Potassium channels propagate electrical signals, maintain membrane potentials and facilitate numerous downstream cellular processes. KirBac3.1 adopts the canonical fold of a K+ channel, with inner and outer membrane-spanning helices supporting an inclined, shorter, pore helix that supports the signature selectivity filter. All feature an hourglass-like constriction at the intracellular opening, leading to the widespread conclusion that the canonical permeation gate at the helix bundle crossing is closed (or nearly so) in all Kir structures, whether determined by crystallography or single-particle cryo-EM. Thus, data presented here indicate that inward rectifiers (Kir) are able to conduct without requiring the substantial conformational changes predicted by the canonical gating mechanism.

To covalently constrain the dimensions of the hourglass-like constriction, paired cysteine point mutants were introduced into KirBac3.1 upon a cysteine-less background, in which each of the three native cysteine residues were substituted for serine or valine (C262S, C71V, C119V). This allowed us to covalently link the four inner helices into a tetramer without obstructing the conduction pathway. Following purification of A133C-T136C and S129C-F135C, covalent linkages between adjacent subunits were generated, either by direct disulfide formation using Cu2+ as the oxidant or by the crosslinking reagents 1,1-methanediyl bismethanethiosulfonate (MTS-1-MTS), which forms compact linkages (CysS–S–CH2–S–SCys) with slightly more tolerance than direct disulfides (CysS–SCys), and dibromobimane, a rigid bicyclic molecule. To visually inspect the channels for intact crosslinks or unanticipated effects on structure, crystal structures of two of the KirBac3.1 adducts, S129C-F135C-MTS-1-MTS and A133C-T136C-bimane were determined. In both mutants, four crosslinks encircle the conduction pathway at the Tyr132 as anticipated. Both revealed electron density bridging between adjacent inner helices, consistent with the predicted covalent linkages. An overlay of both crosslinked structures onto the native pore is illustrated. The cysteine-pair mutants were assayed under identical experimental conditions to wild type. All eight variants of the S129C-F135C or A133C-T136C mutants, either with reduced cysteine sulfhydryl moieties or as covalently-linked adducts with inner helices tethered at Tyr132, mediated K+ movement out of liposomes, with no significant difference in signal from wild type in any of the crosslinked populations, indicating that crosslinking did not prevent K+ flux through the Kir channels. The differences in rate (and overall signal) between crosslinked and reduced forms of the pore are not significant, which indicates the enforced constriction is not rate limiting.

>MTGGMKPPARKPRILNSDGSSNITRLGLEKRGWLDDHYHDLLTVSWPVFITLITGLYLVTNALFALAYLAVGDVIENARPGSFTDAFFFSVQTMATIGYGKLIPIGPLANTLVTLEALVGMLGLAVAACLIYARCTRPTAGVLFSSRMVISDFEGKPTLMMRLANLRIEQIIEADVHLVLVRSEISQEGMVFRRFHDLTLTRSRSPIFSLSWTVMHPIDHHSPIYGETDETLRNSHSEFLVLFTGHHEAFAQNVHARHAYSSDEIIWGGHFVDVFTTLPDGRRALDLGKFHEIAQHHHHHH[2x]> SDNIFV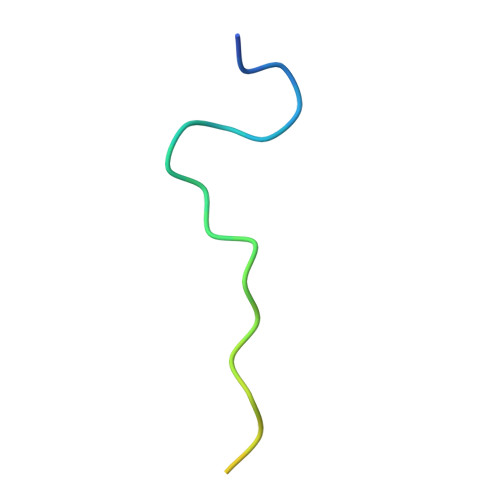KPGEDLEIPLLSDYSDSENISEKS> AQNNPYLFRSNKFLTLFKNQHGSLRLLQRFNEDTEKLENLRDYRVLEYCSKPNTLLLPHHSDSDLLVLVLEGQAILVLV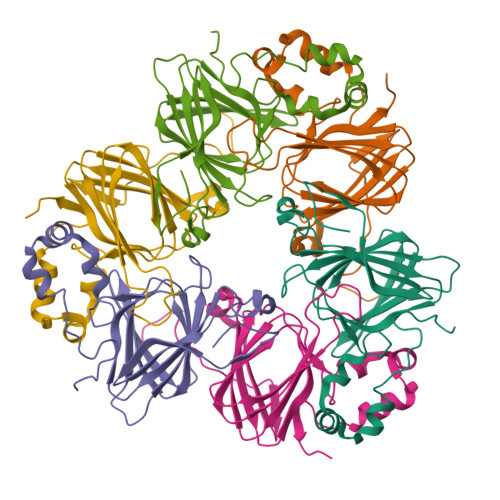NPDGRDTYKLDQGDAIKIQAGTPFYLINPDNNQNLRILKFAITFRRPGTVEDFFLSSTKRLPSYLSAFSKNFLEASYDSPYDEIEQTLLQEEQEGVIVKMPK;> TLSSQDKPFNLRSRDPIYSNNYGKLYEITPEKNSQLRDLDILLNCLQMNEGALFVPHYNSRATVILVANEGRAEVELVGLEQQQQQGLESMQLRRYAATLSEGDIIVIPSSFPVALKAASDLNMVGIGVNAENNERNFLAGHKENVIRQIPRQVSDLTFPGSGEEVEELLENQKESYFVDGQPR> GMQEHYQPAAIEPAAQKKWDDARISNVSEDASKPKYYCLSMFPYPSGKLHMGHVRNYTIGDVLSRFKLLNGFNVMQPMGWDAFGMPAENAAMKNNVAPAAWTYDNIEYMKTQLKSLGFAVDWEREVATCKPEYYRWEQWLFTKLFEKGIVYRKNGTVNWDPVDQTVLANGQVIDGRGWRSGALIEKREIPMYYFKITDYAEELLNDLDKLEHWPEQ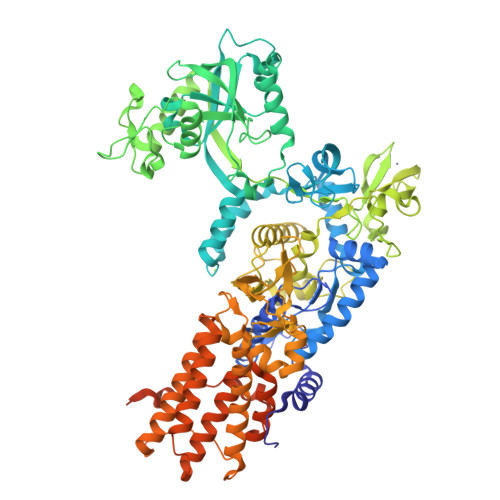VKTMQRNWIGKSRGMTVRFAVSDDSKQGLEGDYAKFLQVYTTRPDTLMGATYVAVAAEHPLATAAAADKPELQAFIAECKAGSVAEADMATMEKKGVPTGRYVVNPLNGDKLEVWIANYVLWGYGDGAVMAVPAHDERDFEFAAKYNLPKKQVIAVGDNAFDANRWQEWYGDKENGVLVNSGDLDGLDFQTAFDAVAAKLQSQGAGEPKTQYRLRDWGISRQRYWGCPIPIVHCEKCGNVPVPADQLPVVLPENVVPDGMGSPLAKMPEFYETSCPCCGGAAKRETDTMDTFIESSWYFFRYMSPKFSDGMVSAESAKYWGAVDQYIGGIEHAILHLLYARFFTKLMRDEGLVNVDEPFERLLTQGMVVCETYYRENDKGGKDWINPADVELTFDDKGRPVSAVLKADGLPVVISGTEKMSKSKNNGVDPQELINAYGADTARLFMMFAAPPEQSLEWSDSGVEGAHRFLRRLWRTVYEYLKQGGAVKAFAGNQDGLSKELKDLRHKLHSTTAKVSDDYGRRQQFNTAIAAVMELLNQYDKTDTGSEQGRAVAQEVLEAAVRLLWPIVPHICETLWSELNGAKLWEAGWPTVDEAALVKSEIEVMVQVNGKLRGKITVAADASKADLEAAALANEGAVKFMEGKPAKKIIVVPGRLVNIVV{(E)-2-[6-(acetylamino)-8-(naphthalen-1-yl)quinolin-2-yl]ethenyl}phosphonic 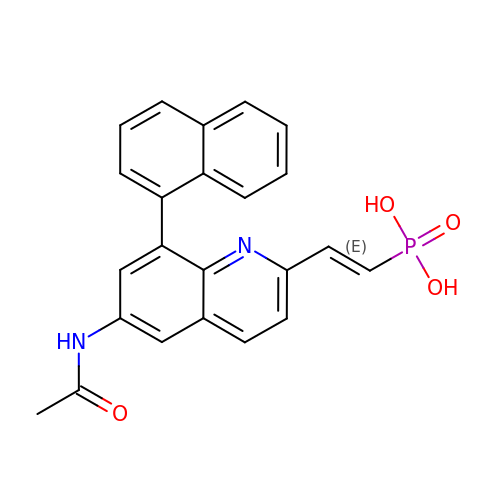acid | C23 H19 N2 O4 P | YXNCZDLAUQFYPO-VAWYXSNFSA-N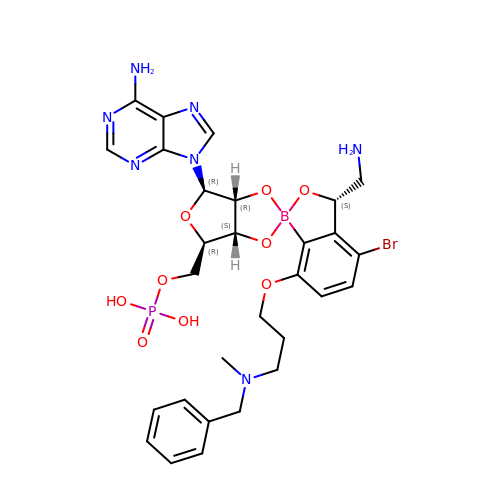[(1R,3'S,5S,6R,8R)-3'-(aminomethyl)-8-(6-aminopurin-9-yl)-4'-bromanyl-7'-[3-[methyl-(phenylmethyl)amino]propoxy]spiro[2,4,7-trioxa-3$l^{4}-borabicyclo[3.3.0]octane-3,1'-3H-2,1$l^{4}-benzoxaborole]-6-yl]methyl dihydrogen phosphate | C29 H35 B Br N7 O9 P | OOVYGSSPEYCEFD-LIBJEQSZSA-N>MKNWKTSAESILTTGPVVPVIVVKKLEHAVPMAKALVAGGVRVLEVTLRTECAVDAIRAIAKEVPEAIVGAGTVLNPQQLAEVTEAGAQFAISPGLTEPLLKAATEGTIPLIPGISTVSELMLGMDYGLKEFKFFPAEANGGVKALQAIAGPFSQVRFCPTGGISPANYRDYLALKSVLCIGGSWLVPA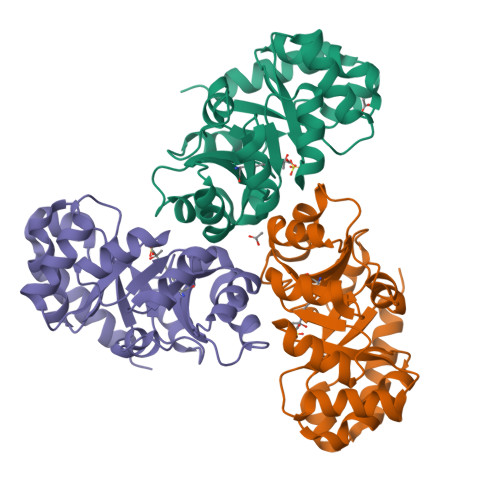DALEAGDYDRITKLAREAVEGAKL[3x]> AVNGKGMNPDYKAYLMAPLKKIPEVTNWETFENDLRWAKQNGFYAITVDFWWGDMEKNGDQQFDFSYAQRFAQSVKNAGMKMIPIISTHQCGGNVGDDCNVPIPSWVWNQKSDDSLYFKSETGTVNKETLNPLASDVIRKEYGELYTAFAAAMKPYKDVIAKIYLSGGPAGALRYPSYTTSDGTGYPSRGKFQAYTEFAKSKFRLWVLNKYGSLNEVNKAWGTKLISELAILPPSDGEQFLMNGYLSMYGKDYLEWYQGILENHTKLIGEL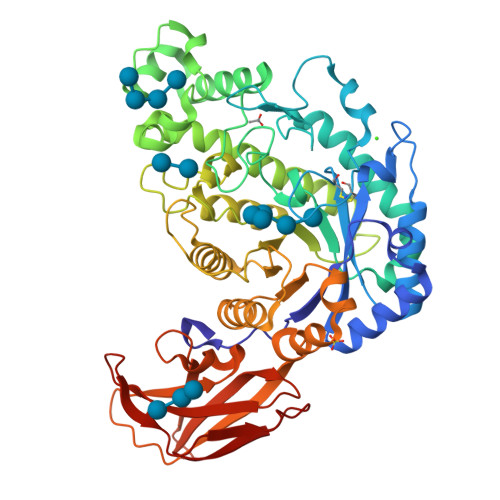AHNAFDTTFQVPIGAKIAGVHWQYNNPTIPHGAEKPAGYNDYSHLLDAFKSAKLDVTFTCLEMTDKGSYPEYSMPKTLVQNIATLANEKGIVLNGENALSIGNEEEYKRVAEMAFNYNFAGFTLLRYQDVMYNNSLMGKFKDLLGVTPVMQTIVVKNVPTTIGDTVYITGNRAELGSWDTKQYPIQLYYDSHSNDWRGNVVLPAERNIEFKAFIKSKDGTVKSWQTIQQSWNPVPLKTTSHTSSW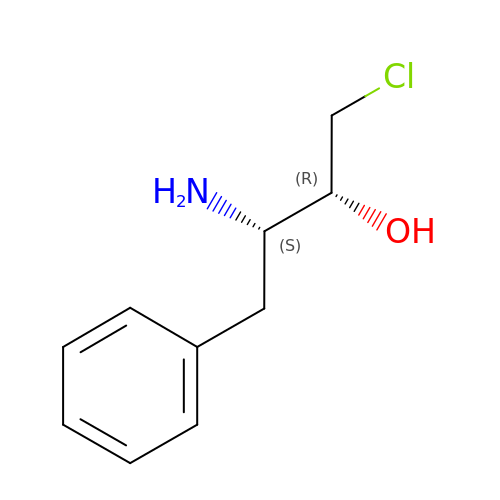(2R,3S)-3-AMINO-1-CHLORO-4-PHENYL-BUTAN-2-OL | C10 H14 Cl N O | YXWOYBQZWSLSMU-UWVGGRQHSA-N>[4x]MAVQPNFLFIFMDDMGWRDLACTGSTFYETPNIDRLCRQGMVFANSYASCPVCSPSRASYLTGQYPARLGVTDWIDMEGTSHPLRGKLIDAPYIKHLPEGEYTIAQALKDAGYETWHVGKWHLGGREYYPDHFGFDVNIGGCSWGHPHEGYFSPYGIETLPEGPEGEYLTDRITDEAVRLLKERKAGGSRKPFYMNLCHYAVH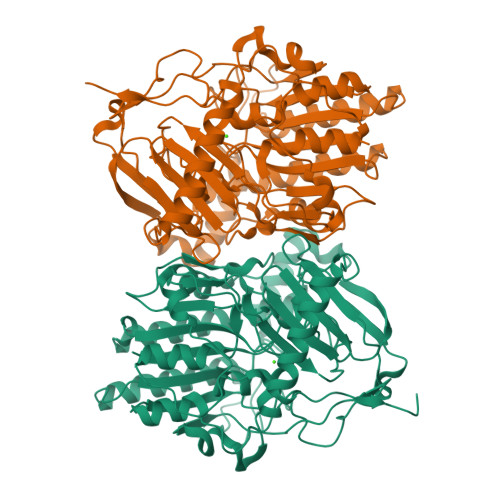TPIQVKDEDRERFEKKAREQGLDQETALVEGEFHHTEDKKGRRVVRRVIQSDPSYAGMIWNLDQNIGRLLEALSECGEEENTVVVFTSDNGGLATSEGSPTCNLPASEGKGWVYEGGTRVPLIVKYPGHVAPGSRCDVPVTTPDFYPTFLELAGVPQKSGIPIDGRSIVPLLAGNHMPERPVFWHYPHYGNQGGTPAASVVLGDYKYIEFFEDGRGELYDLKADFSETNNICENMPEMAARLRMLLHGWQREVCARFPEVNEAYGEV> PLGSMAAGVLKDPEIAD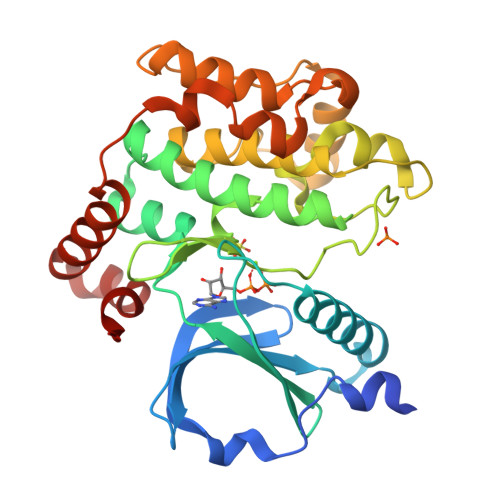LFYKDDPEELFIGLHEIGHGSFGAVYFATNAHTSEVVAIKKMSYSGKQTHEKWQDILKEVKFLRQLKHPNTIEYKGCYLKEHTAWLVMEYCLGSASDLLEVHKKPLQEVEIAAITHGALHGLAYLHSHALIHRDIKAGNILLTEPGQVKLADFGSASMASPANSFVGTPYWMAPEVILAMDEGQYDGKVDIWSLGITCIELAERKPPLFNMNAMSALYHIAQNDSPTLQSNEWTDSFRRFVDYCLQKIPQERPTSAELLRHDFVRRDRPLRVLIDLIQRTKDAVRELDNLQYRKMKKILFQET>[2x]MASGMTVTDAGADQPIVFVNRAFSTITGYAPNEVLGRNARFLQGPQTDAATVARLREAIAAARPIQERILNYRKDGQPFWNQLSISPVRDETGNVVAFVGVQTDVTAHHHHHH

Flavin-binding fluorescent proteins (FbFPs), engineered from prokaryotic and eukaryotic light, oxygen, voltage (LOV) photoreceptors, are promising fluorescent reporter proteins. Their small size (about 10 kDa for monomeric FbFPs such as the improved LOV (iLOV) protein derived from Arabidopsis thaliana phototropin photoreceptors) and their oxygen-independent fluorescence make them ideal reporters to monitor transport and anaerobic biological processes. In contrast to GFP-like fluorescent reporter proteins, whose absorption and fluorescence maxima can be tuned by exchanging certain chromophore-constituting amino acids, the absorption and fluorescence of FbFPs and other flavoproteins depends on noncovalently bound flavins, whose structure cannot be influenced by mutation. Using spectroscopy, X-ray crystallography, and quantum mechanics molecular mechanics calculations, we provide a firm structural and functional understanding of spectral tuning in FbFPs.

To rule out that the I52T mutation alone is sufficient to generate the observed red-shift, we introduced the I52T mutation in parental CagFbFP (light red solid line). The resulting variant showed nearly identical spectral properties as parental CagFbFP (gray dashed line). The latter is corroborated by the X-ray structure of CagFbFP-I52T (see Table S1 for data and refinement statistics), which is virtually identical to parental CagFbFP (C-α atom RMSD 0.52 Å, 102 aligned residues).> MSFSQAVSGLNAAATNLDVIGNNIANSATYGFKSGTASFADMFAGSKVGLGVKVAGITQDFTDGTTTNTGRGLDVAISQNGFFRLVDSNGSVFYSRNGQFKLDENRNLVNMQGMQLTGYPATGTPPTIQQGANPAPITIPNTLMAAKSTTTASMQINLNSTDPVPSKTPFSVSDADSYNKKGTVTVYDSQGNAHDMNVYFVKTKDNEWAVYTHDSSDPAATAPTTASTTLKFNENGILESGGTVNITTGTINGATAATFSLSFLNSMQQNTGANNIVATNQNGYKPGDLVSYQINNDGTV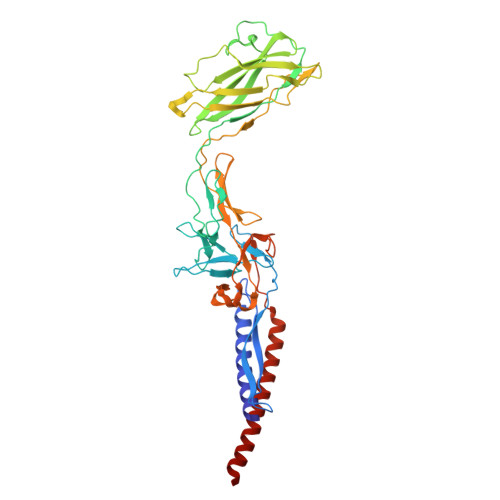VGNYSNEQEQVLGQIVLANFANNEGLASQGDNVWAATQASGVALLGTAGSGNFGKLTNGALEASNVDLSKELVNMIVAQRNYQSNAQTIKTQDQILNTLVNLR> GTCTG;> AGGACTA;> CACCT;> T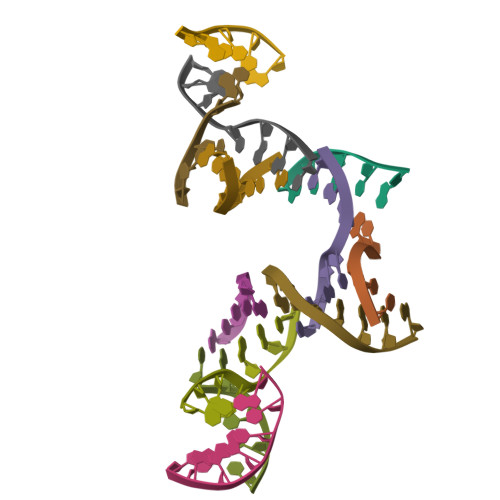AGTGAC The L-arginine biosynthesis pathway consists of eight enzymes that catalyse the conversion of L-glutamate to L-arginine, appears to be attractive target for anti-Tuberculosis (TB) drug discovery. The arginine biosynthesis pathway consists of eight different enzymes ([Fig fig1]) all considered to be essential for *M. tuberculosis* growth *in vitro*. In this work, the ligandability of four enzymes of the pathway ArgB, ArgC, ArgD and ArgF is explored using a fragment-based approach. In conclusion, using a fragment-based approach, we have discovered inhibitors that bind to novel sites in ArgB and ArgF and to the active sites of ArgC and ArgD, which in case of ArgB show on target activity against *M. tuberculosis*.

ArgF displayed a melting temperature of 65.5 °C with 1 mM L-ornithine and L-citrulline showing a positive melting shift of 1.5 and 1 °C respectively. Binding of carbamoyl phosphate to ArgF slightly displaces α-helix 2 when compared to the apo structure. Three X-ray crystal structure of ArgF in complex with different fragments were superposed with the apo structure to create this figure. All fragments keep α-helix 2 in a position close to the apo structure or move further away from the position this helix occupies when carbamoyl phosphate is bound, albeit very slightly.

>GSVIRHFLRDDDLSPAEQAEVLELAAELKKDPVSRRPLQGPRGVAVIFDKNSTRTRFSFELGIAQLGGHAVVVDSGSTQLGRDETLQDTAKVLSRYVDAIVWRTFGQERLDAMASVATVPVINALSDEFHPCQVLADLQTIAERKGALRGLRLSYFGDGANNMAHSLLLGGVTAGIHVTVAAPEGFLPDPSVRAAAERRAQDTGASVTVTADAHAAAAGADVLVTDTWTSMGQENDGLDRVKPFRPFQLNSRLLALADSDAIVLHCLPAHRGDEITDAVMDGPASAVWDEAENRLHAQKALLVWLLERS[6x]2-(pyridin-3-yl)-N-(5-{4-[(5-{[(pyridin-3-yl)acetyl]amino}-1,3,4-thiadiazol-2-yl)amino]piperidin-1-yl}-1,3,4-thiadiazol-2-yl)acetamide | C23 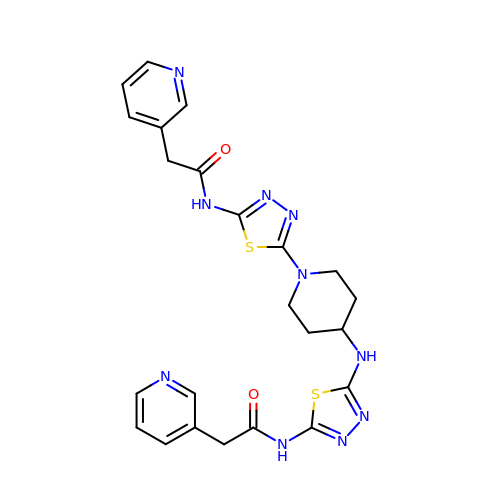H24 N10 O2 S2 | UQDLJRCGWUXXGY-UHFFFAOYSA-N> EAPRHSDWQ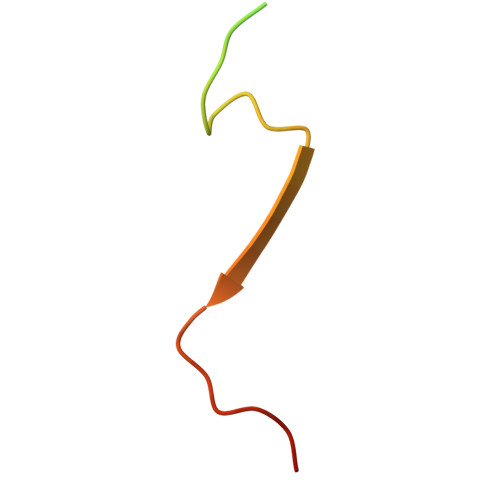RPTFAFEGKGAAGGHTATHHASAAPARPQPVE> PLGSQTTHELTIPNNLIGCIIGRQGANINEIRQMSGAQIKIANPVEGSSGRQVTITGSAASISLAQYLINARLSSEKGMG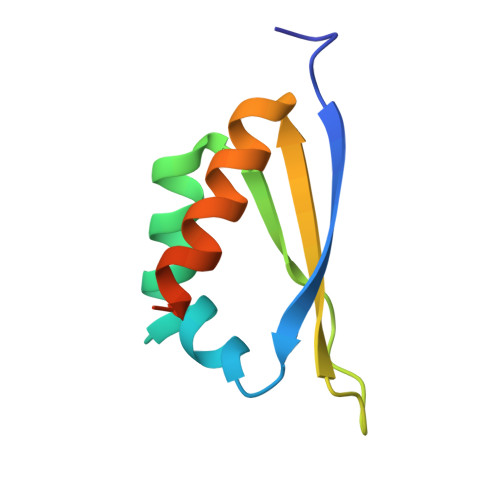CS>[2x]GSHNMAEMVETVCGPVPVEQLGKTLIHEHFLFGYPGFQGDVTRGTFREDESLRVAVEAAEKMKRHGIQTVVDPTPNDCGRNPAFLRRVAEETGLNIICATGYYYGGEGAPPYFQFRRLLGTAEDDIYDMFMAELTEGIADTGIKAGVIKLASSKGRITEYEKMFFRAAARAQKETGAVIITHTQEGTMGPEQAAYLLEHGADPKKIVIGHMCGNTDPDYHRKTLAYGVYIAFDCFGIQGMVGAPTDEER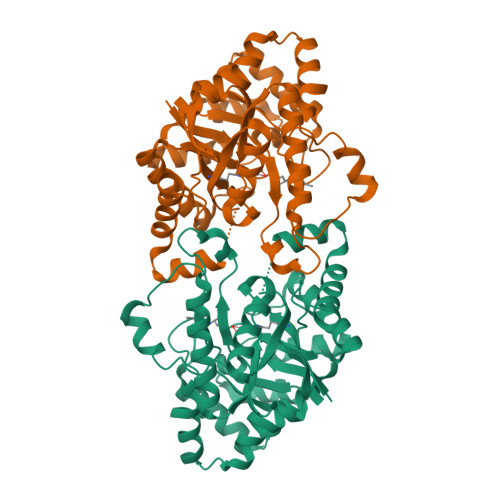VRTLLALLRDGYEKQIMLSHNTVNVWLGRPFTLPEPFAEMMKNWHVEHLFVNIIPALKNEGIRDEVLEQMFIGNPAALFSA> MGRIGILGAGLAGLAAATKLAEAGENVTVFEARNRPGGRVWSETLDTPKGSYVIERGAEFVLDGYTSMRRLLSQFGLSLVDTGMSYYVREPGDTTGITCDDIIRTGREALELASGSGLQGTAEELLAKLPDEPELVDALRARIEISTAVSASEVTARSLQHIASFEPKPSWRVAGGNQRLPDAMAAALGSAVRYGETVRAVENISDGGVLVTTDTDTSVFDTVVVALPLAVIRDSQLNLPTTEARDAALKHVLQGHAAKLHLPLETQPATSAVMSVEGRYWTWTATDESGAVAPVLNAFMGSPSAITRANLKQRPAEWVAKARALRTDLAIPQDAAALTTVWSEDQLAGGAYAAHAPGVTAAGTALLEKPVGDVFWAGEYSEPEFVGLMEGAIRSGERAAGRVMQR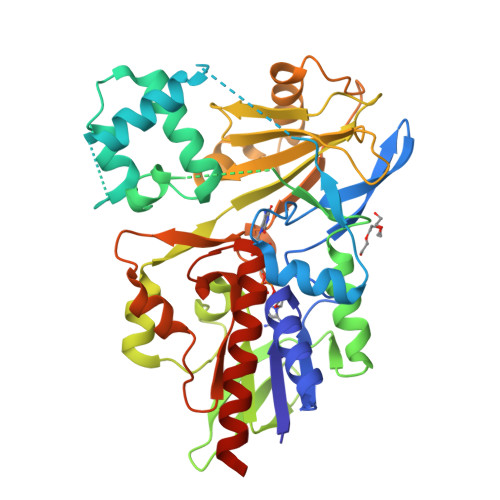LETKSGNSDSERSKA Vaccinia virus, the vaccine used to eradicate smallpox, has about 200 genes, and many of these encode proteins that help the virus evade the host's immune defences. This paper concerns the vaccinia virus proteins A52 and B14, which block signalling pathways leading to the activation of the NF-κB transcription factor and thereby diminish the host immune response to infection. The structures of A52 and B14 are entirely α helical, both comprising seven α helices and adopting the Bcl-2–like fold. We show that both proteins are Bcl-2 family members but lack a surface groove for binding BH3 peptides and, consonant with this, are not anti-apoptotic. Instead these proteins have acquired the ability to inhibit signalling pathways that activate NF-κB.

A52R is an immediate-early VACV gene encoding a 23-kDa intracellular protein (A52) that contributes to virus virulence. A52 functions by inhibiting NF-κB activation downstream of the IL-1 receptor and TLRs via interactions with IRAK2 and TRAF6. The structures of two independent crystal forms of an N-terminal truncated form of A52 comprising residues 37–190 (A52ΔN36) were refined to 1.9 Å and 2.8 Å resolution with residuals R/Rfree = 0.177/0.215 and 0.181/0.192, respectively, with residues 40–189 being observed in electron density maps in both crystal forms. Residue 190 and the first two residues of the polyHis purification tag were also visible in the low-resolution structure. Both crystal forms of A52 contain 2 molecules per asymmetric unit arranged as a dimer, the overall fold (0.32±0.07 Å root-mean-squared displacement [rmsd] over 150 Cα atoms) and dimer interface being highly conserved. To test whether the N terminus of A52, predicted to be unstructured and removed for crystallisation, is required for anti–NF-κB activity, full length A52 and the A52ΔN36 truncation were compared for their ability to block signalling induced by IL-1α. A52ΔN36 had a comparable inhibitory effect to the full-length protein, indicating that the N-terminal 36 residues are not necessary for the inhibitory action of A52. Residues 125–135 of A52, which encompass the 11-residue ‘P13’ peptide sequence that in isolation can inhibit NF-κB activation, form the surface loop between helices 4 and 5. This is distal to the A52 dimerisation interface and is appreciably different in length, amino acid composition and conformation to the comparable loops in the other VACV Bcl-2–like proteins. Residues 92–94 and 117–122 block the groove in A52, the C-terminal ends of helices 2 and 4 being oriented closer to each other than in M11, thereby narrowing the groove significantly, and the side chains of Q93, F94 and Y118 pointing directly into and filling the groove.

>MTDVIKPDYLEYDDLLDRDEMFTILEEYFMYRGLLGLRIKYGRLFNEIKKFDNDAEEQFGTIEELKQKLRLNSEEGADNFIDYIKVQKQDIVKLTVYDCISMIGLCACVVDVWRNEKLFSRWKYCLRAIKLFINDHMLDKIKSILQNRLVYVEMSKHHHHHH[2x]The biosynthesis of the lincosamide antibiotics lincomycin A and celesticetin involves the pyridoxal-5′-phosphate (PLP)-dependent enzymes LmbF and CcbF, which are responsible for bifurcation of the biosynthetic pathways. Despite recognizing the same S-glycosyl-l-cysteine structure of the substrates, LmbF catalyses thiol formation through β-elimination, whereas CcbF produces S-acetaldehyde through decarboxylation-coupled oxidative deamination. To understand the molecular basis for the differences between LmbF and CcbF, we solved the X-ray crystal structures of LmbF and CcbF with PLP at resolutions of 1.7 Å and 1.8 Å, respectively. In the active sites of LmbF and CcbF, the PLP is covalently bound to the catalytic Lys270 and Lys260 residues, respectively, to form internal aldimines.

Although the residues lining the active-site cavity are in comparable positions, Asn205, Phe236, Leu83′ and Pro302′ in LmbF are uniquely substituted with Tyr195, Tyr226, Tyr72′ and Tyr292′ in CcbF, respectively. In CcbF, His76 interacts with the amide of the substrate, and Trp140 and Asp141 form a hydrogen-bond network with the carboxylate of the cysteine moiety, maintaining an ~90° dihedral ψ angle between the Cα–COO− bond and the pyridine ring of PLP. The PPL moiety of 4 is flexible and located at the entrance of the active site, which is consistent with the substrate tolerance of CcbF. These differences in the binding modes of the cysteine moiety would allow CcbF to catalyse decarboxylation as the first step in the enzyme reaction. As a result, the LmbF-like conformation is thought to be a non-reactive binding mode in CcbF. These in silico analyses suggest that the active-site Trp140 and the Tyr72′, Tyr195, Tyr226 and Tyr292′ residues in CcbF play important roles in substrate binding and selectivity in the first step of the enzyme reaction. The LmbF-like conformation is not stable in CcbF due to interactions between the carboxylate of 4 and Tyr72′, Tyr195 and Tyr226, as well as the steric hindrance among the octose and Tyr72′ and Tyr292′. Interactions of the carboxylate with Trp140 align the Cα–COO− bond parallel to the p orbital of the pyridine ring, enabling decarboxylation to form the quinonoid intermediate. Afterwards, due to the absence of a proton donor residue, the quinonoid intermediate donates an electron to an oxygen molecule to generate the semiquinone radical and superoxide. Interestingly, although CcbF has four tyrosine residues in the active site, the Cα of the quinonoid intermediate is isolated from these tyrosines to prevent its protonation. Tyr195 in CcbF is crucial for the selectivity of the first reaction step through steric effects with the Cα-carboxylate, and the Y195G variant favours decarboxylation-coupled oxidative amidation to produce 9. Furthermore, the CcbF Y72L/Y195G/Y226F and Y72L/Y195G/Y292A variants, containing the mutation of Tyr72′ (Leu83′ in LmbF), catalyse oxygen-independent β-elimination.

>MSDLAAVDDWSTLRRIAIDAVSTGRNPELKWLADHPEGTPAYALHLADPLEGAPEGLRQCLREAWDEPLDSYVLSHHGLPELRQAMERWFADDENWPRRRRLLTTATMTGTGPAMYDLLRTIKAREPEGPMAALVPRPGWDYRLFAHDVGYEPIGYHVPFTSPTGPEPGDLDRAVEQTRAKGLRPTVLVLNPQHYATGGNWTPEFVRYALSLADTLGMWVLVDNAYHGMTAAGTQPTSTVRLALDGGFEERLIHVRTLGKQFACNGWAVGSVTAMPDVIDEFAHRWRGFREYPGHAREQAAFAGWLNNPESRKWADERREAIRSNGDALLDALAEVSNTTRHCHGGSPFVLFEVPGGWSQEDFRQRLFADTGVLLASAQIPYAPDWVKVFLGRRPDRFLPAVEALRTRPSRAWQPRLEHHHHHHHH[4x]>MGGYFLDTPKFKRLPGHIAIIPDGNRRWALDRGLEKHEGYKHGIVPGLELYDICVKIGIGEVTFFGFTQDNTKRPQIQRKAFVDACIKSVKELSKHDAELLVVGNTNSDMFPKELLAYTKRTKFGKGKVRINFLVNYGWYWDLTYAFENSSDSKKMIENIASAEIPRID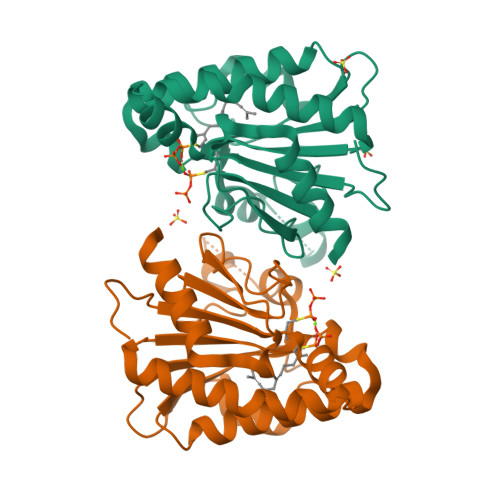LLIRWGGRRRLSGMLPVQTVYSDIYVVDEMWPDFKPEHLFNALEFYQDQDITLGG[2x]4-methyl-2-(2-naphthalen-1-yl-2-oxidanylidene-ethyl)sulfanyl-1~{H}-pyrimidin-6-one 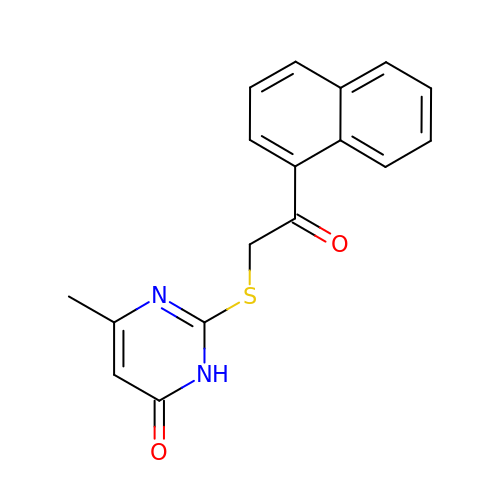| C17 H14 N2 O2 S | KKPLVAUVHOSUPR-UHFFFAOYSA-N>MGQGDESERIVINVGGTRHQTHRSTLRTLPGTRLAWLAEPDAHSHFDYDPRADEFFFDRHPGVFAHILNYYRTGKLHCPADVCGPLYEEELAFWGIDETDVEPCCWMTYRQHRDAEEALDSFGGAPLDNSADDADADGPGDSGDGEDELEMTKRLALSDSPDGRPGGFWRRWQPRIWALFEDPYSSRYARYVAFASLFFILVSITTFCLETHERFNPIVNKTEIENVRNGTQVRYYREAETEAFLTYIEGVCVVWFTFEFLMRVIFCPNKVEFIKNSLNIIDFVAILPFYLEVGLSGLSSKAAKDVLGFLRVVRFVRILRI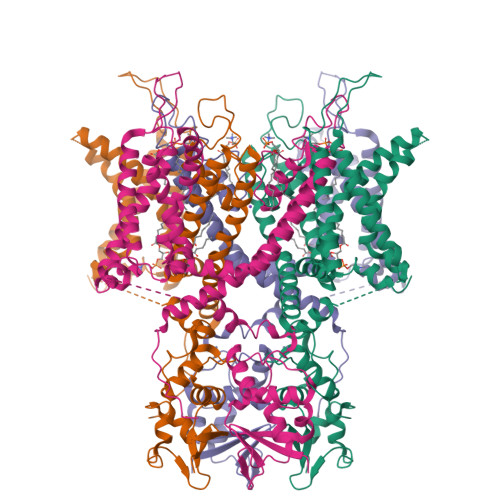FKLTRHFVGLRVLGHTLRASTNEFLLLIIFLALGVLIFATMIYYAERIGAQPNDPSASEHTHFKNIPIGFWWAVVTMTTLGYGDMYPQTWSGMLVGALCALAGVLTIAMPVPVIVNNFGMYYSLAMAKQKLPKKKKKHIPRPPQLGSPNYCKSVVNSPHHSTQSDTCPLAQEEILEINRAGRKPLRGMSIAENLYFQ[4x]1-[[4-[4-[[2-phenyl-5-(trifluoromethyl)-1,3-oxazol-4-yl]carbonylamino]phenyl]phenyl]carbonylamino]cyclopentane-1-carboxylic 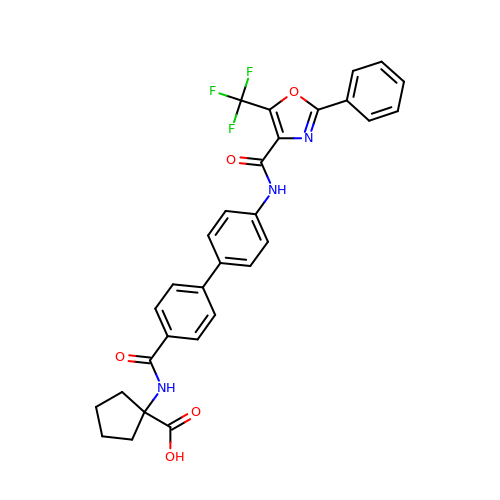acid | C30 H24 F3 N3 O5 | KCKYDKRAHWWVSJ-UHFFFAOYSA-N>[3x]ETVQVNLPVSLEDLFVGKKKSFKIGRKGPHGASEKTQIDIQLKPGWKAGTKITYKNQGDYNPQTGRRKTLQFVIQEKSHPNFKRDGDDLIYTLPLSFKESLLGFSKTIQT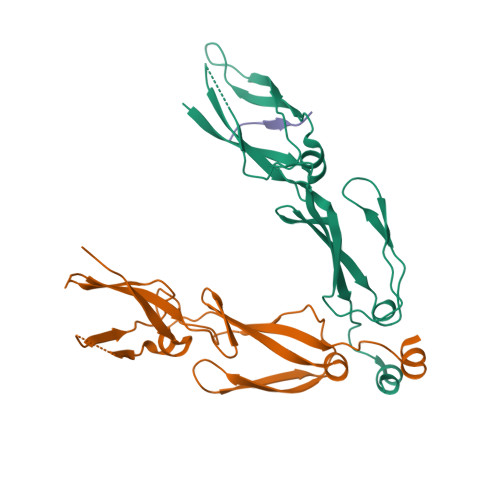IDGRTLPLSRVQPVQPSQTSTYPGQGMPTPKNPSQRGNLIVKYKVDYPISLNDAQKRAIDENF;> PTVEEVD> GEFAQECQNLEVERQRRLERIKQKQSQLQELILQQIAFKNLVQRNRHAEQQASRPPPPNSVIHLPFIIVNTSKKTVIDCSISNDKFEYLFNFDNTFEIHDDIEVLKRMGMACGLESGSCSAEDLKMARSLVPKALEPYVTEMAQGTVGGVFITTA;> GHMREIADKLIELKAEIEELQQREQELDQHKVWVQQSIRNVTEDVQNSCLAYVTHEDICRCFAGDTLL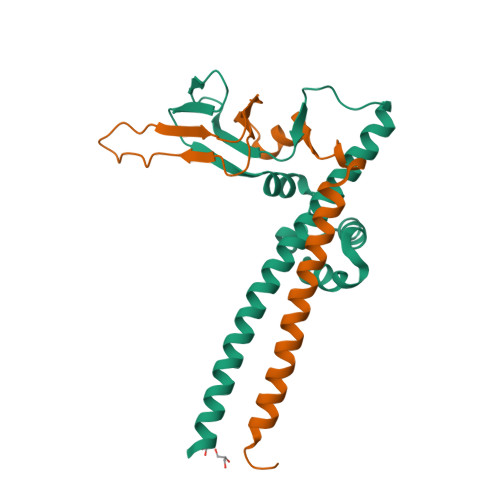AIRAPSGTSLEVPIPEGLNGQKKYQIHLKSVSGPIEVLLVNKE> MVPISPIETVPVKLKPGMDGPKVKQWPLTEEKIKALVEICTEMEKEGKISKIGPENPYNTPVFAIKKKDSTKWRKLVDFRELNKRTQDFWEVQLGIPHPAGLKKKKSVTVLDVGDAYFSVPLDEDFRKYTAFTIPSINNETPGIRYQYNVLPQGWKGSPAIFQSSMTKILEPFAAQNPDIVIYQYMDDLYVGSDLEIGQHRTKIEELRQHLLRWGLTTPDKKHQKEPPFLWMGYELHPDKWTVQPIVLPEKDSWTVNDIQKLVGKLNWASQIYPGIKVRQLSKLLRGTKALTEVIPLTEEAELELAENREILKEPVHGVYYDPSKDLIAEIQKQGQGQWTYQIYQEPFKNLKTGKYARMRGAHTNDVKQLTEAVQKITTESIVIWGKTPKFKLPIQKETWETWWTEYWQATWIPEWEFVNTPPLVKLWYQLEKEPIVGAETFYVDGAANRETKLGKAGYVTNKGRQKVVPLTNTTNQKTELQAIYLALQDSGLEVNIVTDSQYALGIIQAQPDKSESELVNQIIEQLIKKEKVYLAWVPAHKGIGGNEQVDKLV;> PISPIETVPVKLKPGMDGPKVKQWPLTEEKIKALVEICTEMEKEGKISKIGPENPYNTPVFAIKKKDSTKWRKLVDFRELNKRTQDFWEVQLGIPHPAGLKKKKSVTVLDVGDAYFSVPLDEDFRKYTAFTIPSINNETPGIRYQYNVLPQGWKGSPAIFQSSMTKILEPFKKQNPDIVIYQYMDDLYVGSDLEIGQHRTKIEELRQHLLRWGLTTPDKKHQKEPPFLWMGYELHPDKWTVQPIVLP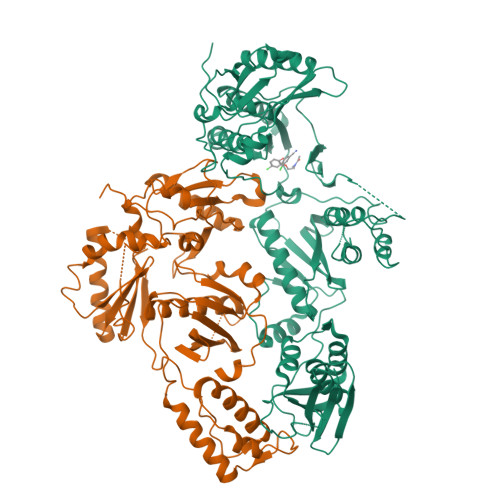EKDSWTVNDIQKLVGKLNWASQIYPGIKVRQLSKLLRGTKALTEVIPLTEEAELELAENREILKEPVHGVYYDPSKDLIAEIQKQGQGQWTYQIYQEPFKNLKTGKYARMRGAHTNDVKQLTEAVQKITTESIVIWGKTPKFKLPIQKETWETWWTEYWQATWIPEWEFVNTPPLVKLWYQ>GSDSGTEEYELNGGLPPGTPGSPDASPARWGWRHGPINVNHYASKKSAAESMLDIALLMANASQLKAVVEQGPSFAFYVPLVVLISISLVLQIGVGVLLIFLVKYDLNNPAKHAKLDFLNNLATGLVFIIVVVNIFITAFGVQKPLMDMAPQQ[6x]

Plasma membrane rupture was long thought to be driven by osmotic pressure, but it has recently been shown to be in many cases an active process, mediated by the protein ninjurin-18 (NINJ1). NINJ1 is a 16-kDa plasma membrane protein that is evolutionarily conserved and found in all higher eukaryotes. Our data thus suggest that, during lytic cell death, the extracellular α-helices of NINJ1 insert into the plasma membrane to polymerize NINJ1 monomers into amphipathic filaments that rupture the plasma membrane. The membrane protein NINJ1 is therefore an interactive component of the eukaryotic cell membrane that functions as an in-built breaking point in response to activation of cell death.

To characterize polymeric NINJ1 at the atomic level, we expressed full-length, wild-type hNINJ1 (residues 1–152) recombinantly in Escherichia coli and extracted it from the bacterial membrane with the detergent n-dodecyl-β-d-maltopyranoside (DDM). The filaments were linear stacks of subunits, with an interval of 20.95 Å and a slight rotation of –1.05° per subunit. The cryo-EM map had a resolution of 3.8 Å, enabling us to build a molecular model of filamentous hNINJ1. The next 103 residues (residues 39–141) were well represented in the maps and could be modelled unambiguously as four α-helices α1–α4. Notably, the experimental density comprised two identical hNINJ1 filaments, which were packed together in an antiparallel arrangement. The hNINJ1 filament is organized by stacking of adjacent protomers in a fence-like manner. The two antiparallel helices α3 and α4 (residues 79–103 and 114–138, respectively) form the core of the filament. The two N-terminal helices α1 and α2 (residues 44–55 and 58–74, respectively) are separated by a distinct kink at L56. α2 thus adopts a parallel orientation with respect to α3 and α4, whereas α1 protrudes at a nearly 90° angle from the helical bundle and connects to the adjacent protomer via an extensive polymerization interface. The intermolecular contacts include multiple side chain interactions between helix α1 of one protomer and helices α1, α3 and α4 of the neighbouring protomer, of which a salt bridge between the highly conserved residues K45 and D53 is the most prominent. When analysing the surface hydrophobicity of the NINJ1 filament, we observed that one face of the filament is hydrophilic whereas the other face is hydrophobic. These properties directly explain how two hNINJ1 filaments have stacked via their hydrophobic faces to result in the soluble double filament resolved by cryo-EM.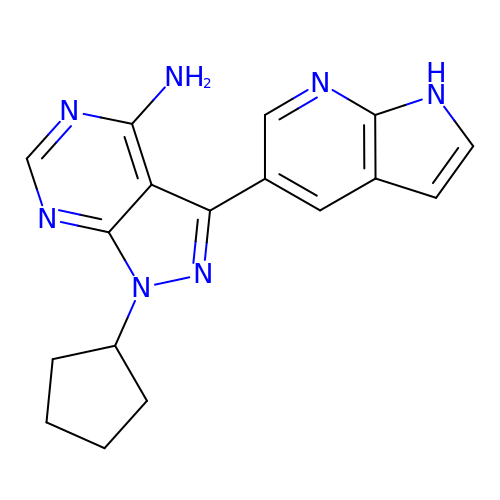1-cyclopentyl-3-(1H-pyrrolo[2,3-b]pyridin-5-yl)-1H-pyrazolo[3,4-d]pyrimidin-4-amine | C17 H17 N7 | NVRXTLZYXZNATH-UHFFFAOYSA-N> MKSVVTTVIAAADAAGRFPSSSDLESVQGSIQRAAARLEAAEKLAGNIDAVATEAYNACIKKYPYLNNAGEANSTDTFKAKCARDIKHYLRLIQYCLVVGGTGPL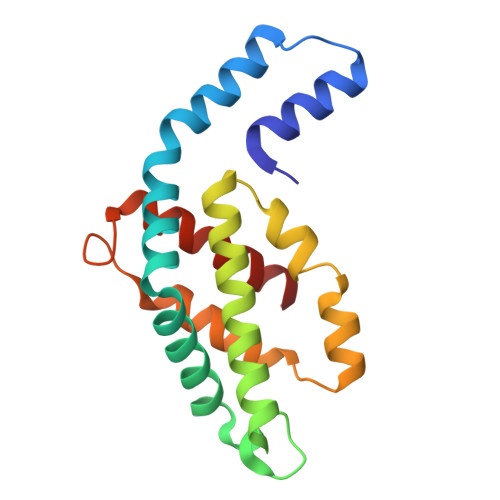DEWGIAGQREVYRALGLPTAPYVEALSFARNRGCAPRDMSAQALTEYNALLDYAINSLS1-[(2S)-4-(7H-PURIN-6-YL)MORPHOLIN-2-YL]METHANAMINE 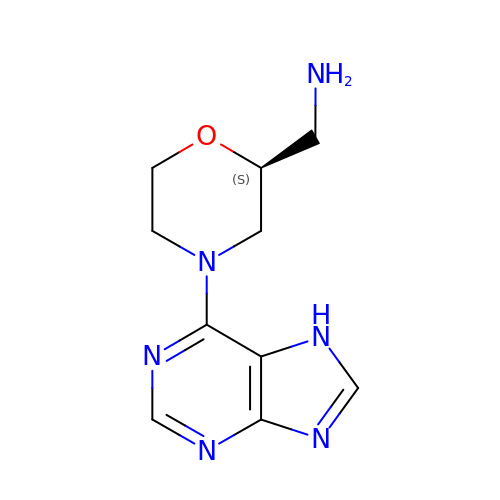| C10 H14 N6 O | VNGSDLIBIYNHKQ-ZETCQYMHSA-N> MATDGLHENETLASLKSEAESLKGKLEEERAKLHDVELHQVAERVEALGQFVMKTRRTLKGHGNKVLCMDWCKDKRRIVSSSQDGKVIVWDSFTTNKEHAVTMPCTWVMACAYAPSGCAIACGGLDNKCSVYPLTFDKNENMAAKKKSVAMHTNYLSACSFTNSDMQILTASGDGTCALWDVESGQLLQSFHGHGADVLCLDLAPSETGNTFVSGGCDKKA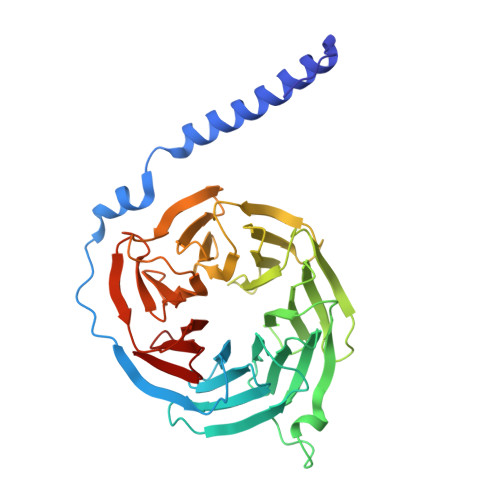MVWDMRSGQCVQAFETHESDVNSVRYYPSGDAFASGSDDATCRLYDLRADREVAIYSKESIIFGASSVDFSLSGRLLFAGYNDYTINVWDVLKGSRVSILFGHENRVSTLRVSPDGTAFCSGSWDHTLRVWA>HMSLVTTSTSDGICTVKINRPDKLNAMNTDVAKELIKTFEELNHNDDVKVIILTGEGEKAFSAGADIEYMSKISADESVEYAKTGQLVTATVELVKQPTIAAVNGFALGGGCELAMSCDIRIAADTAKLGQPEVTIGVPPGWGGTQRLMRIVGIAKA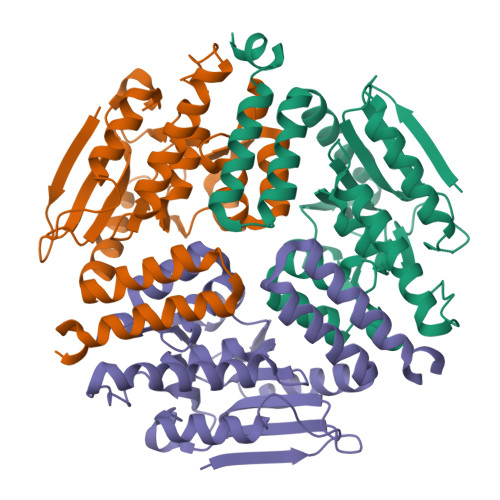KELVYTGKMIKAEEAKEIGLVNHVVPLASLQEEALKMAQQIAGNSTMGVQMSKVAINKGRNADLDTGLGLEILAWRNCFTHPDRQERMT[6x]> MRSSTILQTGLVAALPFAVQAASGSGQSTRYWDCCKPSCSWSGKAPVNRPVLACDANNNPLSDASVKSGCDGGSAYTCANNSPWAVNDQLSYGFAATKLSGGTESSWCCACYALTFTSGPVAGKTLVVQSTSTGGDLGSNHFDINMPGGGVGLFDGCKRQFGGLPG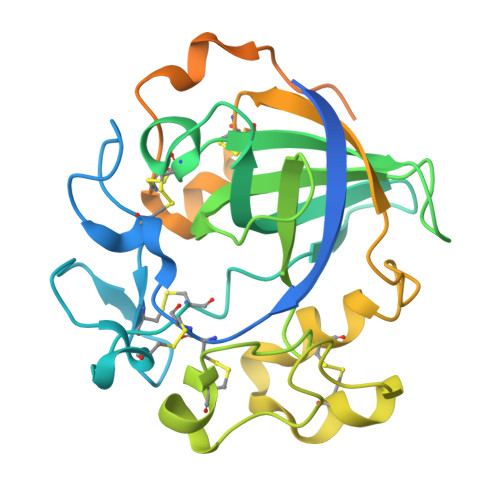AQYGGISSRSQCDSFPAALKPGCQWRFDWFQNADNPNFTFKQVQCPSELTSRTGCKRNDDSQFPVFTPPSGGGSNPSTPTTPPSSGGGSGCTADKYAQCGGSGWSGCTNCPSGSTCKTINDYYHQCA CYCLOHEXYLFORMAMIDE | C7 H13 N O | 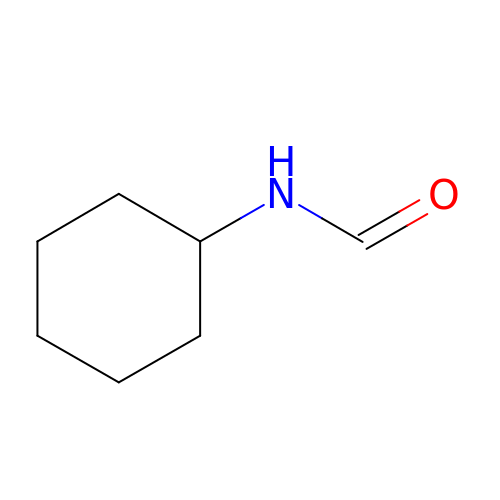SWGXDLRCJNEEGZ-UHFFFAOYSA-N4-({(2S)-2-[2-(4-chlorophenyl)-5,6-difluoro-1H-benzimidazol-1-yl]-2-cyclohexylacetyl}amino)benzoic acid | C28 H24 Cl F2 N3 O3 | 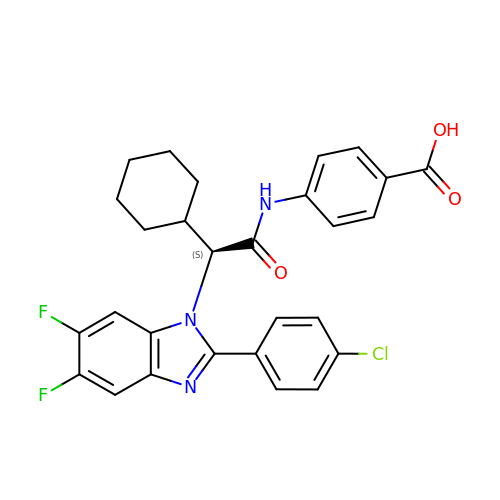OZGKPOZAIWDSQB-VWLOTQADSA-N>[2x]MNTEAEQQLLHHARNGNAEEVRKLLAAMARMEVVADIDCKGRSKSNLGWTPLHLACYFGHKQVVEDLLKAGAKVNMLNDMGDTP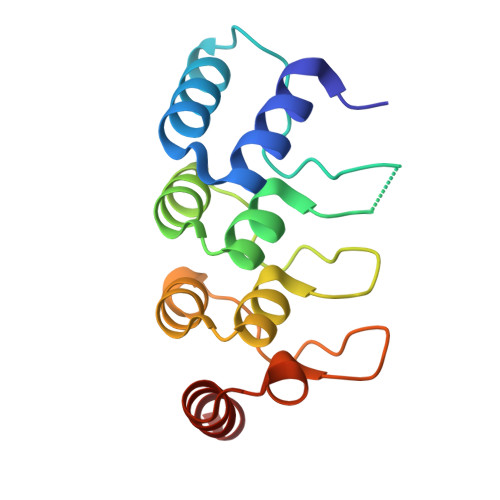LHRAAFTGRKELVLLLLEYDADSTVVNGSGQTAKEATHDKEIRNMLEAVERT NAMPT functions as a homo-dimeric enzyme that catalyzes the rate limiting step in the primary salvage pathway for NAD synthesis, the transfer of a phosphoribosyl residue from 5-phosphoribosyl-1-pyrophosphate (PRPP) to nicotinamide (NAM) to produce nicotinamide mononucleotide (NMN). Crystal structures of NAMPT in numerous ligand-bound forms have been reported. These structures consistently display a NAMPT homo-dimer with two essentially identical active sites at the dimer interface. Typical NAMPT inhibitors were found to occupy the portion of active site responsible for NAM binding and a tunnel-shaped cavity extending from the NAM binding site. Furthermore, we determine the crystal structures of six NAMPT mutants in the apo form and in complex with various inhibitors and present a definitive model to explain the differential effects of the mutations on various structural classes of NAMPT inhibitors.

The crystal structures of G217 mutants revealed that they also perturbed inhibitor binding through a His191-mediated mechanism. Glycine is required for this position to allow a water molecule to bind and participate in the D219-H191-WAT-Y188 network. The addition of a Cβ atom in G217A occludes the water molecule and disrupts the hydrogen bond network. In addition, A217 pushes the H191 imidazole ring away from its normal orientation by 30°, rendering this part of the tunnel less compatible with GNE-618 binding. Similar to H191R, inhibitors with narrow and flexible linkers, including APO866, are less sensitive to the relatively subtle changes induced by the G217A and G217V mutations, which is also consistent with the modest drop in the biochemical potency of compounds 9-11. Compounds with a bulky phenyl group in the core (series A and compound 12) were less active on all G217 mutants, while compounds with a narrow more flexible linker (series B and compound 11) maintain much of their potency on the more conservative changes of G217A and G217V.

>[2x]MNPAAEAEFNILLATDSYKVTHYKQYPPNTSKVYSYFECREKKTENSKLRKVKYEETVFYGLQYILNKYLKGKVVTKEKIQEAKDVYKEHFQDDVFNEKGWNYILEKYDGHLPIEIKAVPEGFVIPRGNVLFTVENTDPECYWLTNWIETILVQSWYPITVATNSREQKKILAKYLLETSGNLDGLEYKLHDFGYRGVSSQETAGIGASAHLVNFKATDTVAGLALIKKYYGTKDPVPGYSVPAAEHSTITAWGKDHEKDAFEHIVTQFSSVPVSVVSDSYDIYNACEKIWGEDLRHLIVSRSTQAPLIIRPDSGNPLDTVLKVLEILGKKFPVTENSKGYKLLPPYLRVIQGDGVDINTLQEIVEGMKQKMWSIENIAFGSGGGLLQKLTRDLLNCSFKCSYVVTNGLGINVFKDPVADPNKRSKKGRLSLHRTPAGNFVTLEEGKGDLEEYGQDLLHTVFKNGKVTKSYSFDEIRKNAQLNIELEAAHHLEHHHHHHHH>MHGSNKLPGFATRAIHHGYDPQDHGGALVPPVYQTATFTFPTVEYGAACFAGEQAGHFYSRISNPTLNLLEARMASLEGGEAGLALASGMGAITSTLWTLLRPGDEVLLGNTLYGCTFAFLHHGIGEFGVKLRHVDMADLQALEAAMTPATRVIYFESPANPNMHMADIAGVAKIARKHGATVVVDNTYCTPYLQRPLELGADLVVHSATKYLSGHGDITAGIVVGSQALVDRIRLQGLKDMTGAVLSPHDAALLMRGIKTLNLRMDRHCANAQVLAEFLARQPQVELIHYPGLASFPQYTLARQQMSQPGGMIAFELKGGIGAGRRFMNALQLFSRAVSLGDAESL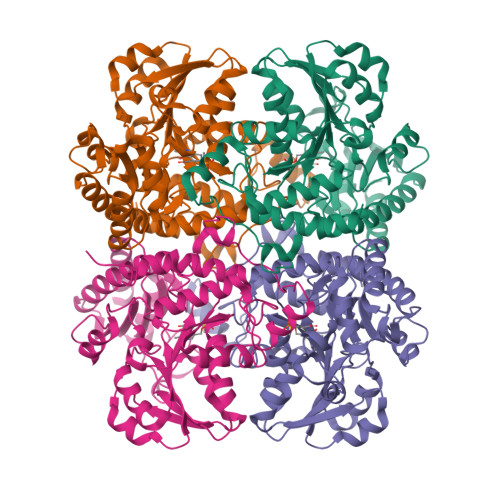AQHPASMTHSSYTPEERAHYGISEGLVRLSVGLEDIDDLLADVQQALKASA[4x]>GPGSFKERRPFHERQKDVEEIRSQQPNKVPVIIERFDGERSLPLMDRCKFL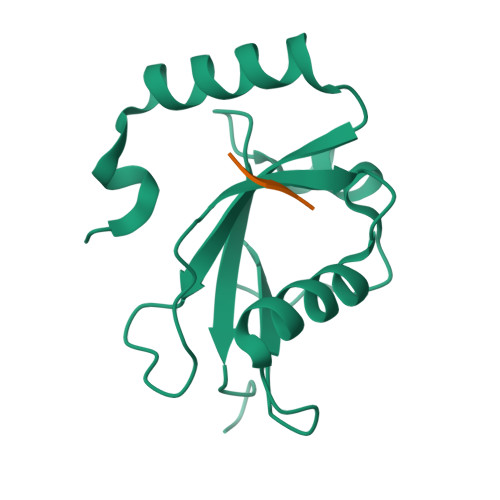VPEHITVAELMSIVRRRLQLHPQQAFFLLVNERSMVSNSMSMSNLYSQERDPDGFVYMVYTSQPAFG[4x];>[4x]WEEL>[2x]VRERGPQRVAAHITGTRGRSNTLSSPNSKNEKALGRKINSWESSRSGHSFLSNLHLRNGELVIHEKGFYYIYSQTYFRFQEEIKENTKNDKQMVQYIYKYTSYPDPILLMKSARNS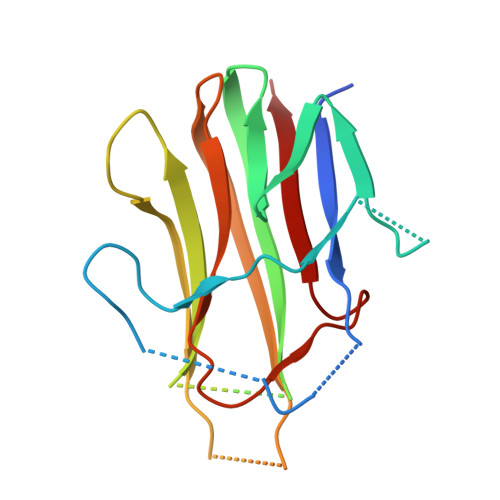CWSKDAEYGLYSIYQGGIFELKENDRIFVSVTNEHLIDMDHEASFFGAFLVG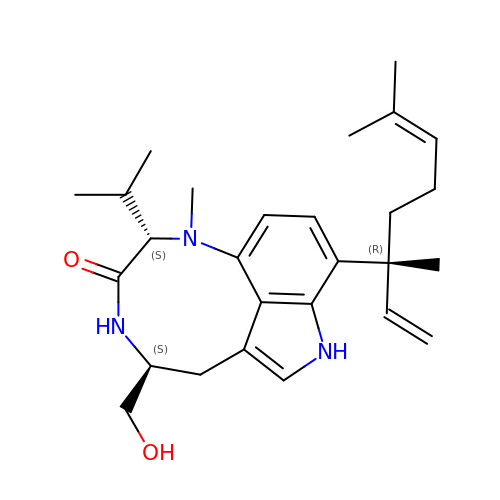(2S,5S)-9-[(3R)-3,7-dimethylocta-1,6-dien-3-yl]-5-(hydroxymethyl)-1-methyl-2-(propan-2-yl)-1,2,4,5,6,8-hexahydro-3H-[1,4]diazonino[7,6,5-cd]indol-3-one | C27 H39 N3 O2 | KISDGNGREAJPQR-OICBGKIFSA-N>MNSKKSPVTLIGLGPMGQAMVRTLLGQGHPVTVWNRTPSRAEPLVVEGARLAASPTEAVASSDLVILSLTDYQAMYDILSTAESALAGRTIVNLSSDDPD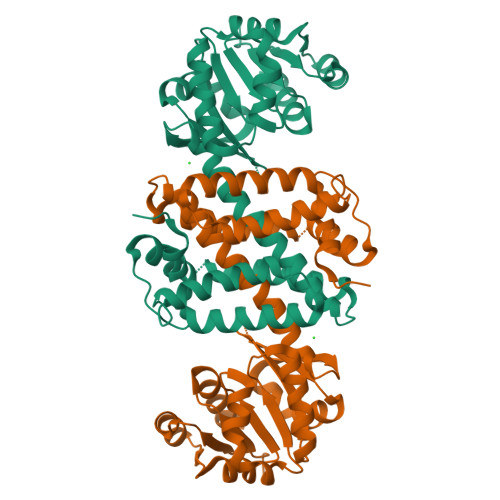VTREAAKWAAKHGATFIAGGVMIPAPTVGTEAAYVFYSGPKSAFDAHEPVLRHIGGPRFLGEDTGLAQLYYLAHLDVLLTTLASVVHATALVSAAGVDEAAFAPEAIRMVIETGQMLAAEAETGLELARNLASGNHPGELATAVMMGATADHIVSAAKGSGVDLVLPEAVKSLYDRTVAAGHGKDSWTAMYEIIKKKAA[3x]>[12x]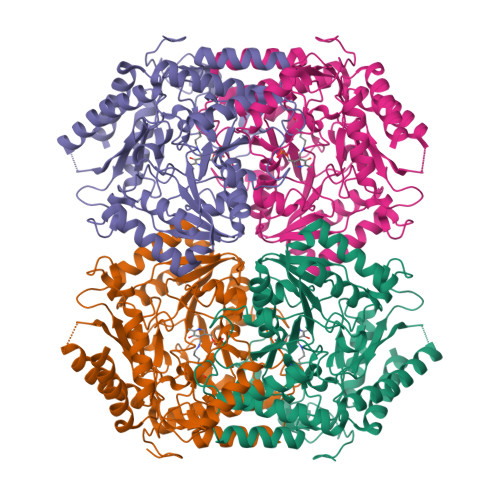MTTTANELSYRIEQKRNINGAFPGPKSQALAERRSAVVAAGVASGVPVYVEDADGGIIRDVDGNSFIDLGSGIAVTSVGASDPAVVAAVQEAAAHFTHTCFMVTPYEGYVAVTEQLNRLTPGDHAKRTVLFNSGAEAVENAVKVARLATGRDAVVAFDHAYHGRTNLTMALTAKAMPYKTNFGPFAPEVYRMPMSYPFREENPEITGAEAAKRAITMIEKQIGGDQVAAIIIEPIQGEGGFIVPAEGFLPALSEWAKEKGIVFIADEVQSGFCRTGEWFAVDHEGVVPDIITMAKGIAGGLPLSAITGRADLLDAVHPGGLGGTYGGNPVACAAALAAIDTMEQHDLNGRARHIEELALGKLRELAAELSAGGGSVVGDIRGRGAMLAIELVQPGSKEPNAELTKAVAAACLKEGVIILTCGTYGNVIRLLPPLVISDELLIDGLEVLAAAIKAHA> MDINDKLSIDSPIDNKNIIEFITFRTDTSGIQKKIKAYQIAKHIWVVPERYYAEPLNISDEYKIDGGIYNENYLTTDKERQEYLDAICILFKRINNVIEGKKLLSLLSSASPFPFKDDTNKYLLKEALLYVNEENFEFKFFTSNIILFGPGTNISKNQVLPLNGDDATSGVGSVSEICYNPFFTKKFGEYSLDPVIGLIECLLKSLYNLYGIKVSDDIKIPYKLQRALNTDKYSYINLEEALIFGGNDYKIFTEKPYWLSNDYFLKSLNTFEENKAKYEKDLKNDPNLNNELNQYLQQKYSFSISKIWSLNLTAFADIFNINIPTSFLASITFWDRSQYYKINYPNDYNIDGFVNGQWNTNLKNIEKDNNFIIFDKPKQIITYINDIFNLRYTSNLYEDNLDIESNNYYLNFMFEYDKGNNFTINQYKALLDTLDNDFIDSLPPIQGMNAQNKLTSLPIISKGTDTENINSELLLPIHYLKSQTYNLDMYSSIKFTTNIYEVVSEKNSELVYTFLPHINEIMENY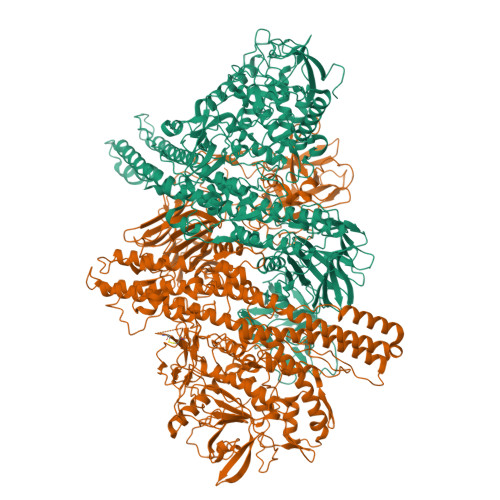SINNTIKTEEEFYNWMENLFINYSIDILEKRNSIIPGITAVLPWIGKALNILNTNNDFEEELQLSGIKGLIKEYENFIIPDMIVPDIPLDNMPRTYDDIDKKLSEIYTKNKFLFLKGYYFIVQEWWTTYYIQFIELKYLCSGAINKQQQLLITVLEKQLFYFTNNGLFPFDAMERMINEFNRSIDIFSRISQQALNNVDIFINECALFIFNNEVYPLFLNNVENNINKANDNVLNYINKATSLTEEQIKELTVKYTFSSIAEVEFFNESYFKKITNMDIKNILTNIKNINNLILSGSQINDDITIFDESGNNLNIKFDPSIRIVDGHTNVAFKLDKSSQYINIPTENINFSFMESFSIDFWLKILDSTESTTLLNCIEDDIGWKLSIQNNNLLWEMKDNLGNNFTSLFTFNINNIWHNITLSIDRLTNTFNCFLDGKLINTDNISNIFSLETNTPIEIQSDNGAILLEAFSILNYPLQQQEVLNRYREAFSNNYTRNYYGDILKYNENYQLYNKTSPDKEVKKVFTNDKDYIAIEYNQNTNNPTFFSLIQKEQSKIYVEENDEVYICVQGDPLNYITIDNNQAVLTKDINLATSFKLKTNLNKPNSLIFSENSQALRLSNRLNDENYILLDLVSKLDDEPLNIFYWEFI;> MKLEINKFNYNDPIDGINVITMRPPRHSDKINKGKGPFKAFQVIKNIWIVPERYNFTNNTNDLNIPSEPIMEADAIYNPNYLNTPSEKDEFLQGVIKVLERIKSKPEGEKLLELISSSIPLPLVSNGALTLSDNETIAYQENNNIVSNLQANLVIYGPGPDIANNATYGLYSTPISNGEGTLSEVSFSPFYLKPFDESYGNYRSLVNIVNKFVKREFAPDPASTLMHELVHVTHNLYGISNRNFYYNFDTGKIETSRQQNSLIFEELLTFGGIDSKAISSLIIKKIIETAKNNYTTLISERLNTVTVENDLLKYIKNKIPVQGRLGNFKLDTAEFEKKLNTILFVLNESNLAQRFSILVAKHFLKERPIDPIYVNILDDNSYSTLEGFNISSQGSNDFQGQLLESSYFEKIESNALRAFIKICPRNGLLYNAIYRNSKNYLNNIDLEDKKTTSKTNVSYPCSLLNGCIEVENKDLFLISNKDSLNDINLSEEKIKPETTVFFKDKLPPQDITLSNYDFTEANSIPSISQQNILERNEELYEPIRNSLFEIKTIYVDKLTTFHFLEAQNIDESIDSSKIRVELTDSVDEALSNPNKVYSPFKNMSNTINSIETGITSTYIFYQWLRSIVKDFSDETGKIDVIDKSSDTLAIVPYIGPLLNIGNDIRHGDFVGAIELAGITALLEYVPEFTIPILVGLEVIGGELAREQVEAIVNNALDKRDQKWAEVYNITKAQWWGTIHLQINTRLAHTYKALSRQANAIKMNMEFQLANYKGNIDDKAKIKNAISETEILLNKSVEQAMKNTEKFMIKLSNSYLTKEMIPKVQDNLKNFDLETKKTLDKFIKEKEDILGTNLSSSLRRKVSIRLNKNIAFDINDIPFSEFDDLINQYKNEIEDYEVLNLGAEDGKIKDLSGTTSDINIGSDIELADGRENKAIKIKGSENSTIKIAMNKYLRFSATDNFSISFWIKHPKPTNLLNNGIEYTLVENFNQRGWKISIQDSKLIWYLRDHNNSIKIVTPDYIAFNGWNLITITNNRSKGSIVYVNGSKIEEKDISSIWNTEVDDPIIFRLKNNRDTQAFTLLDQFSIYRKELNQNEVVKLYNYYFNSNYIRDIWGNPLQYNKKYYLQTQDKPGKGLIREYWSSFGYDYVILSDSKTITFPNNIRYGALYNGSKVLIKNSKKLDGLVRNKDFIQLEIDGYNMGISADRFNEDTNYIGTTYGTTHDLTTDFEIIQRQEKYRNYCQLKTPYNIFHKSGLMSTETSKPTFHDYRDWVYSSAWYFQNYENLNLRKHTKTNWYFIPKDEGWDED> MAEEEEVEEGRSSSSAILDLPEPLLLHILSFLTDVRSRHRAALACGRMRAAERATRSELSLRGDPRSPGFLFLSHAFRFPALEHLDLSLVSPWGHPLLSSVPPCGGGGGGAPSASSSSGMNVYHPEAISEQNAFIAARLAGCFPAVTSLAVYCRDPTTLANLTPHWQASLRRVKLVRWHQRPPTLPDGADLEPLLETCAALRELDLSEFYCWTEDVVRALTTHPSATAALTHLDLGLAAATDGFKSSELGPIAASCPNLRKLVAPCLFNPRFSDCVGDDALLSLATSCPRLTVLRLSEPFEAAANIQR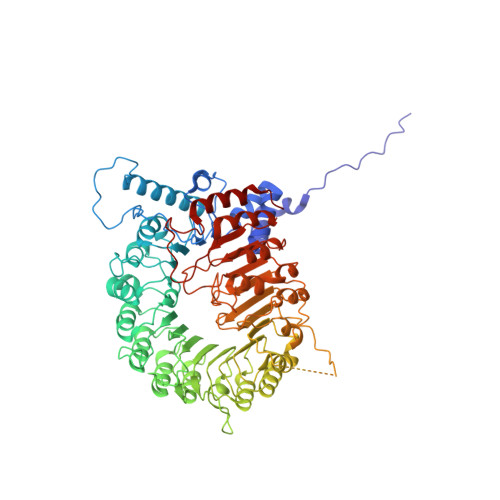EEAAITVAGLVAFFAALPALEDFTMDLQHNVLEAAPAMEALARRCPRIKFLTLGSFQGLCKASWLHLDGVAVCGGLESLYMKNCQDLTDASLAAIGRGCRRLAKFGIHGCDLVTSAGIRRLAFTLRPTLKEVTVLHCRLLHTAECLTALSPIRDRIESLEINCVWNTTEQPCSVANGTTTECDPEDDELGEVYESAAKKCRYMEFDDLGSWEMLRSLSLWFSAGQLLSPLISAGLDSCPVLEEISIKVEGDCRTCPRPAPRTIFGLSDLAGFPVLAKMKLDLSEAVGYALTAPTGQMDLSLWERFYLHGIESLQTLYELDYWPPQDKDVHHRSLTLPAVGLIQRCVGLRKLFIHGTTHEHFMTFFLSIPNLRDMQLREDYYPAPENDLMFTEMRAESWLRFEVQLNSRQIDD>[2x]VFHKIRNEDLIFNESLGQGTFTKIFKGVRREVGDYGQLHETEVLLKVLDKAHRNYSESFFEAASMMSKLSHKHLVLNYGVCVCG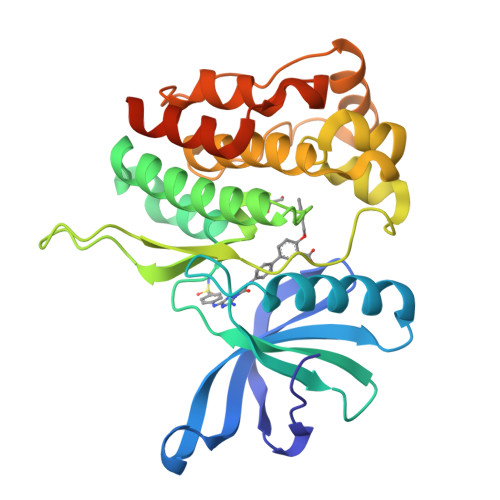DENILVQEFVKFGSLDTYLKKNKNCINILWKLEVAKQLAAAMHFLEENTLIHGNVCAKNILLIREEDRKTGNPPFIKLSDPGISITVLPKDILQERIPWVPPECIENPKNLNLATDKWSFGTTLWEICSGGDKPLSALDSQRKLQFYEDRHQLPAPKAAELANLINNCMDYEPDHRPSFRAIIRDLNSLFTPDLVPRGSHHHHHH3-(2-AMINO-6-BENZOYLQUINAZOLIN-3(4H)-YL)-N-CYCLOHEXYL-N-METHYLPROPANAMIDE | C25 H30 N4 O2 | 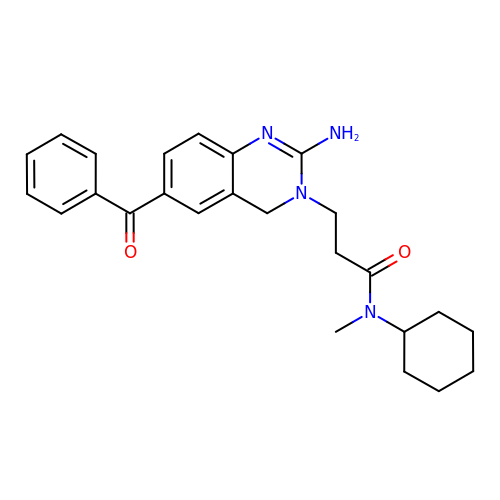KTRFBFMYAJOXLG-UHFFFAOYSA-N> MDKNRVFGQRLRQSIQNYFSSP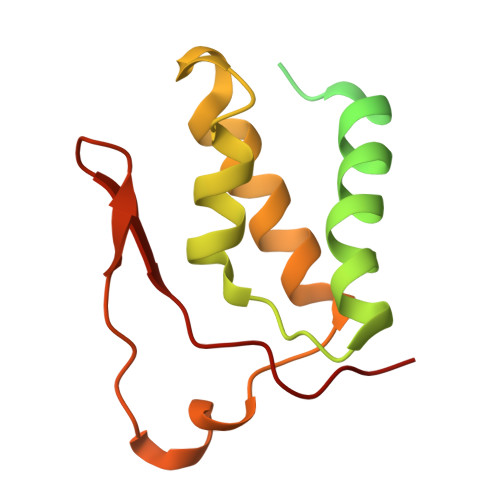WLLYTAKAEALLDLRDDEAMLNEMEAVGELPMALEYESLTDVQTQIVTAIQAELAHFRNTAQPINLGAVLQEQLARYPQSRHFDVARIIVDQAVKLGMASQDHQAVYPVWQPIDDFSAAVQAHLIDQYDK>[2x]AIRVADLLQHITQMKCAEGYGFKEEYESFFEGQSAPWDSAKKDENRMKNRYGNIIAYDHSRVRLQTIEGDTNSDYINGNYIDGYHRPNHYIATQGPMQETIYDFWRMVWHENTASIIMVTNLVE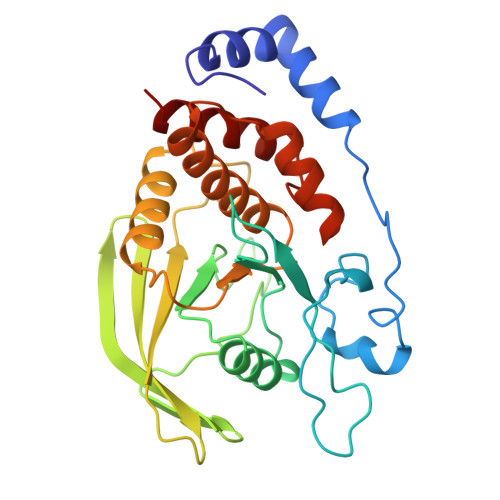VGRVKCCKYWPDDTEIYKDIKVTLIETELLAEYVIRTFAVEKRGVHEIREIRQFHFTGWPDHGVPYHATGLLGFVRQVKSKSPPSAGPLVVHCSAGAGRTGCFIVIDIMLDMAEREGVVDIYNCVRELRSRRVNMVQTEEQYVFIHDAILEACL> MEDKKIVIMPCKCAPSR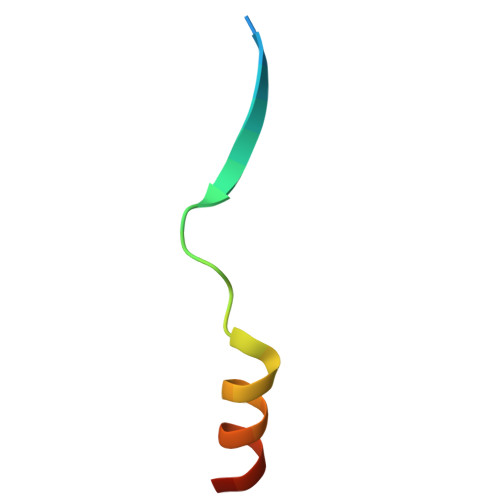QLVQVWLQAKE Acid ceramidase (aCDase; ASAH1) is the best studied member of the family and is prominent for its involvement in Farber disease (FD), a genetic disorder in humans. aCDase is ubiquitously expressed and found in the lysosome where it normally regulates sphingolipid metabolism through intralysosomal membrane turnover. Similar to other Ntn-hydrolases, aCDase is synthesized as an inactive proenzyme that requires proteolysis for activation. The α-subunit consists of a globular helical domain formed by five α-helices preceded by a 36-residue linker region, whereas the β-subunit contains two central anti-parallel β-sheets flanked on either side by a total of six α-helices.

Two structures are of the full-length proenzyme before autocleavage, from naked mole rat (nmr, 83% identity to human) and common minke whale (cmw, 85% identity). The autocleavage reaction was prevented in these structures by mutating the catalytic cysteine residue to alanine (C143A). In the proenzyme structure, the peptide bond between Cys 143 (Ala 143 in the inactivated structures) and residue 142 (methionine in nmr-aCDase and isoleucine in cmw-aCDase) is intact as shown by continuous electron density. Residues 141 and 142 complete the β-strand, which leads into a tight turn preceded by the C-terminal helix-α5 of the putative α-subunit. The presence of an intact junction combined with the orientation of Cys 143 completely sequester it and the scissile peptide bond from the outside environment, confirming that autocleavage must occur intramolecularly. Since both inactive structures are of the C143A mutant, the position of the thiol was not experimentally determined, but we could model it based on energetically accessible cysteine rotamers and their corresponding steric clashes with the protein. In both inactive structures, only one rotamer satisfies these criteria (Rot1). The structure reveals that a possible general base is Arg 159 as it is the only residue close enough to hydrogen bond with the modeled thiol. Thr 141 is conserved across all species of aCDase and W1 is found in both inactive structures determined here, suggesting that it probably plays an important role. In nmr-aCDase, L4-6 forms an extended structure that protrudes ‘outward,’ whereas in cmw-aCDase it flips toward the center of the protein and sits atop the junction between the subunits. Interestingly, the conformation of L4-6 in active human-aCDase is essentially the same as in nmr-aCDase.

> DRHHHHHHKLQHAPPWTEDCRKSTYPPSGPTYRGPVPWYTINLDLPPYKRWHELMVDKGPMLKIIVNSFKNMVNTFVPSGKVMQMVDQKLPDLLGQFSGPYEEEMKGIADVTEIPLGEIISFNIFYELFTMATSIITEDKKGHLLHVRNMDFGIFLGWNINNNTWVITEELKPLTVNLDFQRNSKTVFKATSFAGYVGMLTGFKPGQFSLTLNERFSMNGGYLGLLEWILGKKDASWIGFITRSVLENATSYEEAKNILAKTKLLAPAYFILGGNQSGEGCVITRERKDSLDIYELDPKQGRWYVVQTNYDRWKNPLFLDDRRTPAQTCLKRTTQESLSFATLYDILSTKPVLNKLTVFTALMDVTKNHYEAYLRDCPDPCVGW>SNAMIHGIGVDLIEIDRIQALYSKQPKLVERILTKNEQHKFNNFTHEQRKIEFLAGRFATKEAFSKALGTG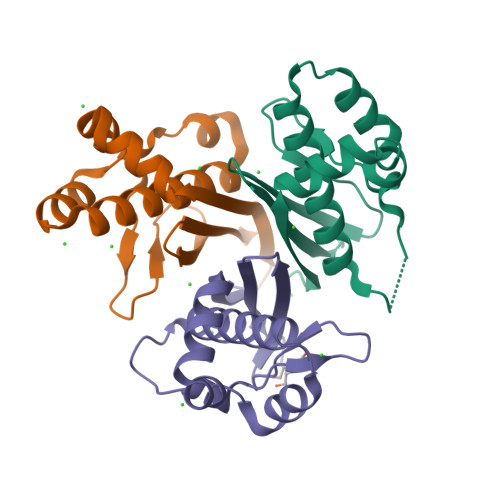LGKHVAFNDIDCYNDELGKPKIDYEGFIVHVSISHTEHYAMSQVVLEKSAF[3x]>SKIYEDNSLTIGHTPLVRLNRIGNGRILAKVESRNPSFSVKCRIGANMIWDAEKRGVLKP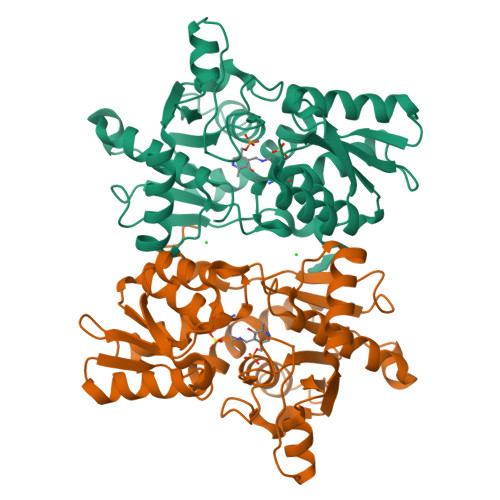GVELVEPTNGNTGIALAYVAAARGYKLTLTMPETMSIERRKLLKALGANLVLTEGAKGMKGAIQKAEEIVASDPQKYLLLQQFSNPANPEIHEKTTGPEIWEDTDGQVDVFISGVGTGGTLTGVTRYIKGTKGKTDLITVAVEPTDSPVIAQALAGEEIKPGPHKIQGIGAGFIPGNLDLKLIDKVVGITNEEAISTARRLMEEEGILAGISSGAAVAAALKLQEDESFTNKNIVVILPSSGERYLSTALFADLFTEKELQQ[4x]>[4x]MGLAQRRMMAEVPNADVIVVNPEHYAVAVKYDVKRSAAPFVIAKGVDDVAFKIREVAREYNIAIVSAPPLARAIYHTTKLDQQIPEGLFTAVAQVL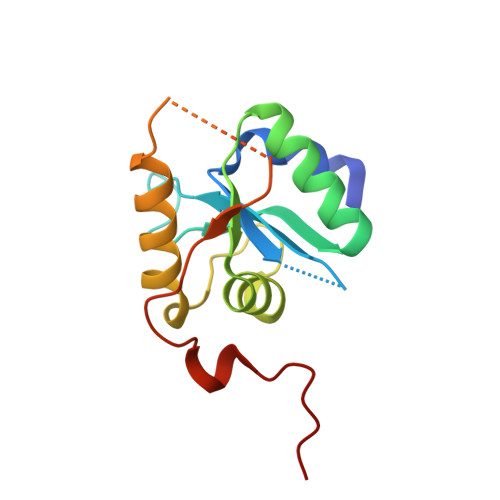AYVFQLRQYQKGRGRKPIPIPLNQPIPDDLKYHHHHHH>MERPQPDSMPQDLSEALKEATKEVHTQAENAEFMRNFQKGQVTRDGFKLVMASLYHIYVALEEEIERNKESPVFAPVYFPEELHRKAALEQDLAFWYGPRWQEVIPYTPAMQRYVKRLHEVGRTEPELLVAHAYTRYLGDLSGGQVLKKIAQKALDLPSSGEGLAFFT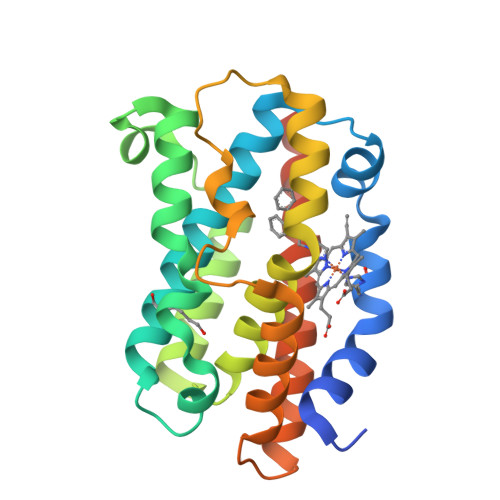FPNIASATKFKQLYRSRMNSLEMTPAVRQRVIEEAKTAFLLNIQLFEELQELLTHDTKDQSPSRA[2x]diethyl ({4-[2-(11-ethyl-5-methyl-6-oxo-6,11-dihydro-5H-dipyrido[3,2-b:2',3'-e][1,4]diazepin-8-yl)ethyl]phenoxy}methyl)phosphonate 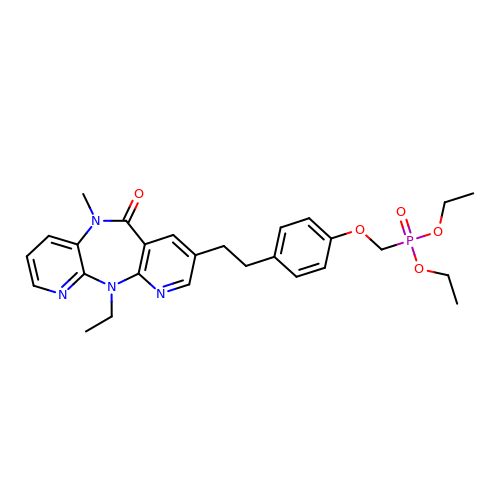| C27 H33 N4 O5 P | YVBXNGRTCURFDW-UHFFFAOYSA-N>[4x]MTHEIKTISVIGATGQQGGSVARSLLQNPEFHVRCITRDTSSIKAKELKELGIEIVQADGNDP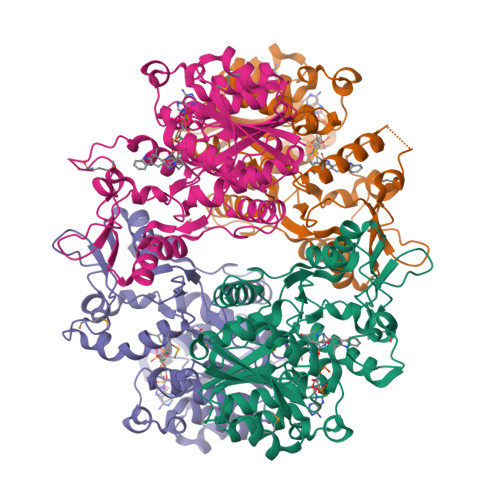TAMATALKGSWGIFINNGYTLTPAVQNGKYEEDFGNVILQSAAEAGVPHVVFSSQPSSHALSGGKFNTPVLDVKAWGESWGRACPTFQSFTPIMASWYFQNFFIPSFVAEFGGFPWNQDDEGYLTLRLPPLGGNEEVPWICIDEDFGDLVHGIFLNPARWSKRTVQAVGDILSYGDLCTTFADVTQRKARYIPYYDLDDMPADRPYLQESRQVFAFYQMRDGELFGNGITEKRTASLLKAAAFQAKGQKGRETLITAREWFERHCRANKTSEKIERSGPIVREDP>DWPVYHRIDGPIVMIGFGSIGRGTLPLIERHFAFDRSKLVVIDPSDEARKLAEARGVRFIQQAVTRDNYRELLVPLLTAGPGQGFCVNLSVDTSSLDIMELARENGALYIDTVVEPWLGFYFDPDLKPEARSNYALRETVLAARRNKPGGTTAVSCCGANPGMVSWFVKQALVNLAADLGVTGEEPTTREEWARLAMDLGVKGIHIAERDTQRASFPKPFDVFVNTWSVEGFVSQGLQPAELGWGTFERWMPDNARGHDSGCGAGIYLLQPGANTRVRSWTPTAMAQYGFLVTHNESISIADFLTVRDAAGQAVYRPTCHYAYHPCNDAVLSLHEMFGSGKRQSDWRILDETEIVDGIDELGVLLYGHGKNAYWYGSQLSIEETRRIAPDQNATGLQVSSAVLAGMVWALENPNAGIVEADDLDFRRCLEVQTPYLGPVVGVYTDWTPLAGRPGLFPEDIDTSDPWQFRNVLVRD[2x]

In contrast to its eukaryotic counterparts, bacterial HSS synthesizes 1 mol HSP from 2 mol PUT. NAD+ serves as a non-covalently bound prosthetic group for BvHSS. The interface area of the dimer was calculated as approximately 1700 Å2 by PDBsum indicating a stable dimer23. The BvHSS subunit consists of two domains as determined by CATH24: one “NAD(P)-binding Rossmann-like” domain (domain 1, residues 3–163 and 394–425) and one “homospermidine-synthase-like domain” (domain 2, residues 164–395 and 426–477) as shown in Fig. 2a and S1. The crystal structures of BvHSS containing NAD+ clearly show that the active site is localized inside each subunit.

Residue Glu-298 has been chosen based on direct interaction with the active site residue His-296, forming a Glu-His-Glu triad together with Glu-237. All four variants of BvHSS lead to enzymatically inactive but soluble enzymes. Other than minimal and most likely negligible rotations of the side chain amide group of amino acid Gln-237 and the side chain of amino acid His-296, no structural changes of active site residues compared with wild-type BvHSS were observed. The exchange of residue Glu-237 by Gln-237 resulted in changes of the electrostatic potential of the surface of the binding pocket. Compared with wild-type BvHSS, because of the change of the pKa value the side chain of His-296 (pKa,calc = 6.4) should no longer be protonated at both nitrogens resulting in a loss of the positive charge at the imidazole ring. Together with the loss of the negative charge of the side chain of residue 237 because of the replacement of glutamate by glutamine, the electrostatic potential of the surface of the pocket inverted at pH 7 and pH 9, at a region around Gln-237, to a now positive electrostatic potential and, at an area around His-296, to a negative electrostatic potential. Of note, the structure of BvHSS variant E237Q does not have PUT bound at the active site neither at the outer nor at the inner binding site. This implies an important role for the residue Glu-237 during substrate binding. Under the assumption that the change of Glu-237 to Gln-237 mimics the electrostatic potential of a fully substrate bound state, the observed rigid and narrow conformation of the pore of the binding pocket supports the concept that it functions as a locking mechanism directed through a substrate-sensing feature of the “track-and-trace” loop. All BvHSS and BvHSS variants co-crystallized with AGM were found to have AGM bound to the protein surface at various sites, most likely causing the observed improvement in crystal growth.Rift Valley fever virus (RVFV; genus phlebovirus, family Phenuiviridae) is an important example of an enveloped virus that harbours a class II fusion protein. As with other phleboviruses, RVFV displays two glycoproteins on the lipid bilayer envelope of the virion, Gn and Gc, which form higher order pentameric and hexameric ring-shaped assemblies. While the Gc glycoprotein is responsible for membrane fusion, the role of the Gn remains undefined. Virus entry is completed upon Gc-mediated fusion of the viral envelope and host cell membrane, in a pH-dependent mechanism.

Localized reconstruction of each of the four types of the Gn–Gc capsomers (pentamers and hexamers of type 1–3) resulted in four independent structures at resolutions between 7.7 and 8.6-Å. Imposing lower than six-fold symmetry (two-fold symmetry for the type 2 hexamer and three-fold symmetry for the type 3 hexamer), or no symmetry (type 1 hexamer) gave the highest resolution, suggesting significant deviations from six-fold symmetry in the hexamers. We first performed fitting with the localized reconstruction of the pentamer at 7.7 Å resolution, followed by fitting the resulting Gn–Gc heterodimer model to localized reconstructions of the hexamers at 8.0–8.6 Å resolution. Consistent with previous biochemical and structural studies, this fitting verified that the Gn and Gc assemble as heterodimers, which form higher order ring-like pentameric and hexameric capsomer structures on the mature virion. Domain A of the Gn forms a ring on top of these capsomers interacting with domain II of Gc, occluding a surface area of ~950 Å2. The Gn–Gc interface is formed between the β-ribbon domain of the Gn and the hydrophobic fusion loops of Gc11, which are shielded from solvent at the interface between Gn domains A and B. Surprisingly, unlike the rod-like array of extended anti-parallel Gc dimers predicted from the low-resolution modelling attempts, we observed that RVFV Gc forms a kinked conformation, not previously sampled in crystallographic investigations of class II fusion glycoproteins. Interestingly, the embedding of the fusion loops was only observed in the case of the pentamers and not with the hexamers.

>EDPHLRNRPGKGHNYIDGMTQEDATCKPVTYAGACSSFDVLLEKGKFPLFQSYAHHRTLLEAVHDTIIAKADPPSCDLQSAHGNPCMKEKLVMKTHCPNDYQSAHYLNNDGKMASVKCPPKYELTEDCNFCRQMTGASLKKGSYPLQDLFCQSSEDDGSKLKTKMKGVCEVGVQALKKCDGQLSTAHEVVPFAVFKNSKKVYLDKLDLKTEENLLPDSFVCFEHKGQYKGKLDSGQTKRELKSFDISQCPKIGGHGSKKCTGDAAFCSAYECTAQYANAYCSHANGSGIVQIQVSGVWKKPLCVGYERVVVKRELS[6x];>DPGCSELIQASSRITTCSTEGVNTKCRLSGTALIRAGSVGAEACLMLKGVKEDQTKFLKIKTVSSELSCREGQSYWTGSFSPKCLSSRRCHLVGECHVNRCLSWRDNETSAEFSFVGESTTMRENKCFEQCGGWGCGCFNVNPSCLFVHTYLQSVRKEALRVFNCIDWVHKLTLEITDFDGSVSTIDLGASSSRFTNWGSVSLSLDAEGISGSNSFSFIESPGKGYAIVDEPFSEIPRQGFLGEIRCNSESSVLSAHESCLRAPNLISYKPMIDQLECTTNLIDPFVVFERGSLPQTRNDKTFAASKGNRGVQAFSKGSVQADLTLMFDNFEVDFVGAAVSCDAAFLNLTGCYSCNAGARVCLSITSTGTGSLSAHNKDGSLHIVLPSENGTKDQCQILHFTVPEVEEEFMYSCDGDERPLLVKGTLIAID[6x]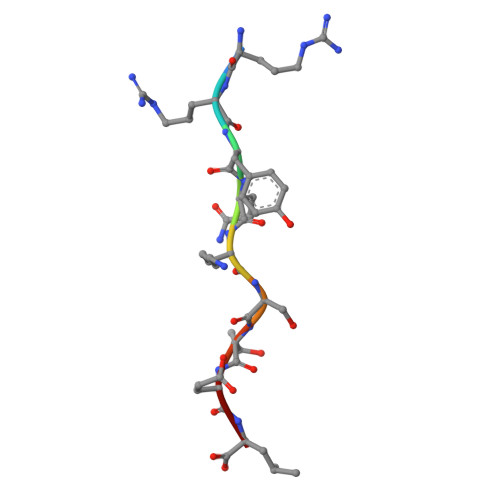> RRYQKSTEL1,2,3-trichloropropane | C3 H5 Cl3 | 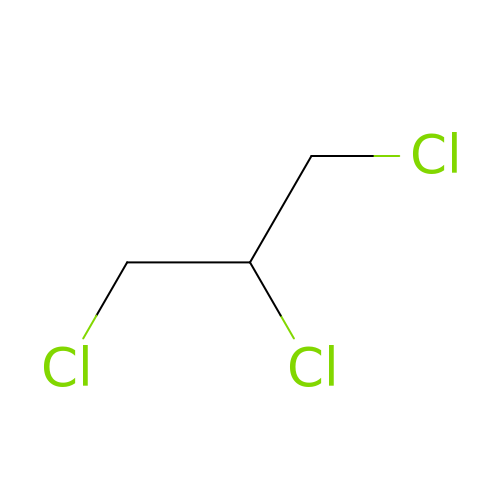CFXQEHVMCRXUSD-UHFFFAOYSA-N> TD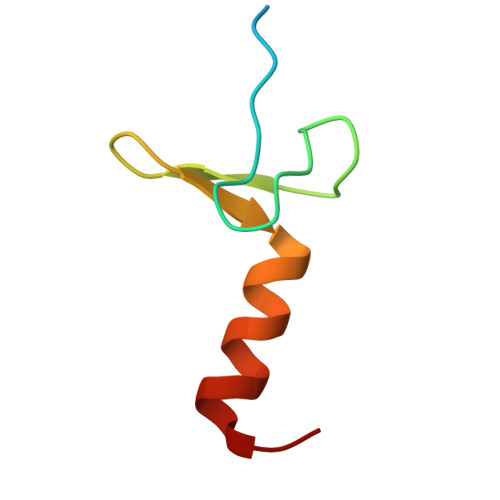KRKDGSGKLLYCSFCGKSQHEVRKLIAGPSVYICDECVDLCNDIIREEI>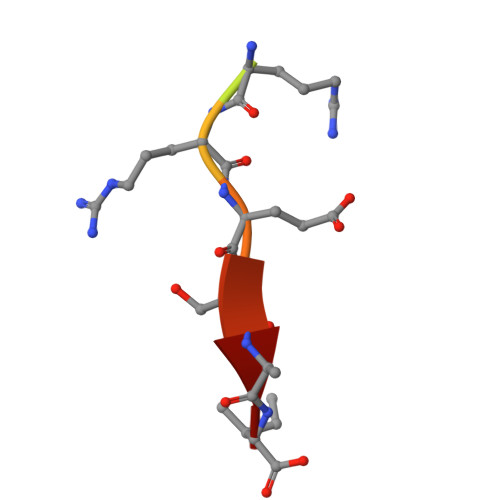 NISYRRESAI> GPGSMNYISTRGAGIGERHTFSDILLGGLAKDGGLYLPSEYPQVSADELARWRTLPYADLAFEILSKFCDDIAAADLRAITRRTYTADVYRHARRGGNAADITPLTTLGTENGAPVSLLELSNGPTLAFKDMAMQLLGNLFEYTLAKHGETL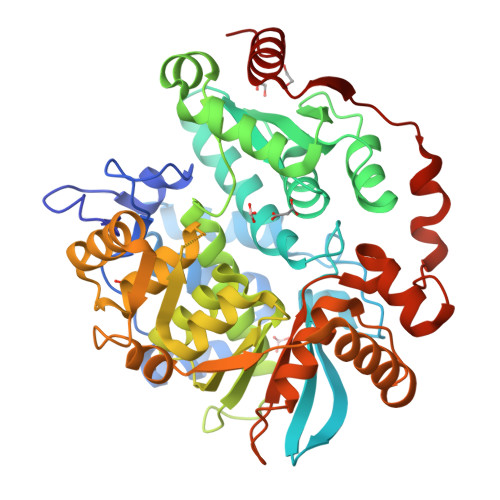NILGATSGDTGSAAEYAMRGKEGVRVFMLSPHKKMSAFQTAQMYSLQDPNIFNLAVNGVFDDCQDIVKAVSNDHAFKAQQKIGTVNSINWARVVAQVVYYFKGYFAATRSNDERVSFTVPSGNFGNVCAGHIARMMGLPIEKLVVATNENDVLDEFFRTGAYRVRSAQDTYHTSSPSMDISKASNFERFVFDLLGRDPARVVQLFRDVEQKGGFDLAASGDFARVAEFGFVSGRSTHADRIATIRDVFERYRTMIDTHTADGLKVAREHLRPGVPMVVLETAQPIKFGESIREALGQEPSRPAAFDGLEALPQRFEVVDANAQQVKDFIAAHTGA> MVPISPIETVPVKLKPGMDGPKVKQWPLTEEKIKALVEICTEMEKEGKISKIGPENPYNTPVFAIKKKDSTKWRKLVDFRELNKRTQDFWEVQLGIPHPAGLKKKK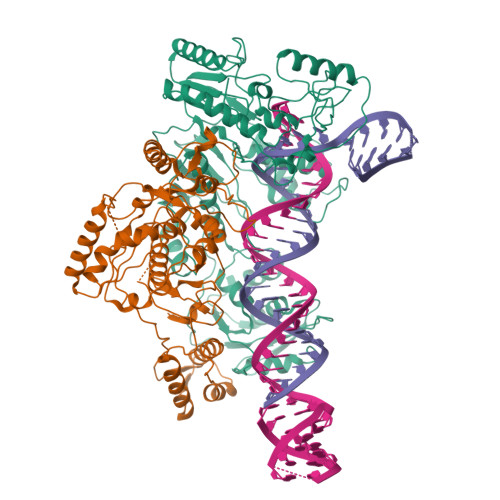SVTVLDVGDAYFSVPLDEDFRKYTAFTIPSINNETPGIRYQYNVLPQGWKGSPAIFQSSMTKILEPFKKQNPDIVIYQYMDDLYVGSDLEIGQHRTKIEELRQHLLRWGLTTPDKKHQKEPPFLWMGYELHPDKWTVQPIVLPEKDSWTVNDICKLVGKLNWASQIYPGIKVRQLSKLLRGTKALTEVIPLTEEAELELAENREILKEPVHGVYYDPSKDLIAEIQKQGQGQWTYQIYQEPFKNLKTGKYARMRGAHTNDVKQLTEAVQKITTESIVIWGKTPKFKLPIQKETWETWWTEYWQATWIPEWEFVNTPPLVKLWYQLEKEPIVGAETFYVDGAANRETKLGKAGYVTNKGRQKVVPLTNTTNQKTQLQAIYLALQDSGLEVNIVTDSQYALGIIQAQPDKSESELVNQIIEQLIKKEKVYLAWVPAHKGIGGNEQVDKLVSAGIRKILDLGTLVPR;> MVPISPIETVPVKLKPGMDGPKVKQWPLTEEKIKALVEICTEMEKEGKISKIGPENPYNTPVFAIKKKDSTKWRKLVDFRELNKRTQDFWEVQLGIPHPAGLKKKKSVTVLDVGDAYFSVPLDEDFRKYTAFTIPSINNETPGIRYQYNVLPQGWKGSPAIFQSSMTKILEPFKKQNPDIVIYQYMDDLYVGSDLEIGQHRTKIEELRQHLLRWGLTTPDKKHQKEPPFLWMGYELHPDKWTVQPIVLPEKDSWTVNDIQKLVGKLNWASQIYPGIKVRQLSKLLRGTKALTEVIPLTEEAELELAENREILKEPVHGVYYDPSKDLIAEIQKQGQGQWTYQIYQEPFKNLKTGKYARMRGAHTNDVKQLTEAVQKITTESIVIWGKTPKFKLPIQKETWETWWTEYWQATWIPEWEFVNTPPLVKLWYQLEKEPIVGAETF>[2x]MAHHHHHHHRSGNLTGKTALVTGASRGIGRAIAEKLGYAGALVAVHYATGADAAAEVAESIEKDGGRAFTVKAELGVPGDVDVLFEGLERGLKERTGATDLDILVNNAGVMAMGAPEEVTPEMFDRMMAVNAKAPFFIVQ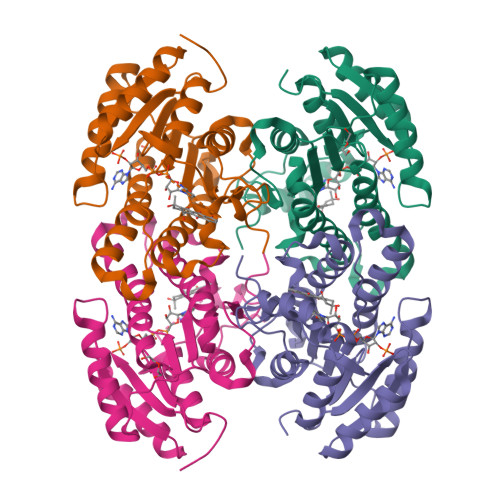RALSVMPDGGRIINVSSGLTRVASPDQVTYGMSKGALEQIALHFSRHLGSRRITVNSVAPGSTDNGSALFQIPEVRETLSQLSTFGEVAEPAAIADVVAFLASEDARWITGAFIDASGGTLLG> UUCCAGUGCGGAGUCUGGAGACACCCAGGGGGAAGCGAAGACCCUAUGGAGCUUUACUGCAGGCUGUCGCUGAGACGUGGUCGCCGAUGUGCAGCAUAGGUAGGAGACACUACACAGGUACCCGCGCUAGCGGGCCACCGAGUCAACAGUGAAAUACUACCCGUCGGUGACUGCGACUCUCACUCCGGGAGGAGGACACCGAUAGCCGGGCAGUUUGACUGGGGCGGUACGCGCUCGAAAAGAUAUCGAGCGCGCCCUAUGGCUAUCUCAGCCGGGACAGAGACCCGGCGAAGAGUGCAAGAGCAAAAGAUAGCUUGACAGUGUUCUUCCCAACGAGGAACGCUGACGCGAAAGCGUGGUCUAGCGAACCAAUUAGCCUGCUUGAUGCGGGCAAUUGAUGACAGAAAAGCUACCCUAGGGAUAACAGAGUCGUCACUCGCAAGAGCACAUAUCGACCGAGUGGCUUGCUACCUCGAUGUCGGUUCCCUCCAUCCUGCCCGUGCAGAAGCGGGCAAGGGUGAGGUUGUUCGCCUAUUAAAGGAGGUCGUGAGCUGGGUUUAGAC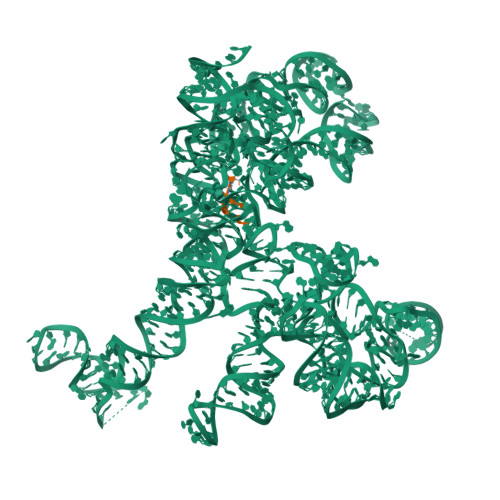CGUCGUGAGACAGGUCGGCUGCUAUCUACUGGGUGUGUA;> CCAA> MAKKTSSKGKLPPRVPNLIPYVGSFVSFAKNPVQFIIDNSKKYGDVFTATILGKEMTFLNHPKILDTFFKATDNELSLRDVYRFMRPVFGTGVVYDADSTERMMEQVKFVSSGLTTARFRVFVDIFEDEIAHKVKELGPEGTVDVAELMADLIIFTASRCLLGDEVRQYLSEKNLGKLYHDIDDGISPLSFFYPSLPAPKRDKARKAVGEIFQELLDKRREEHKKHPERLLDESKMDVVDHLLTQKYKDGQELTDVHRIGILIAGLFAGQHTSSITSSWTLMNVISNKKVLEKVRKEQEEIMGSDKVLDYDKVMKMDYLEACMKEALRMYPPLIMIMRMARKPRECEQYIIPKGNILVVSPSVAGRCTDTYTNPDVFDPERLTERKEHEKFKYGAVPFGAGRHKCIGENFALLQVKSIISILLRYFDMEYIGKIPDPSYTSLVVGPSPPTRMR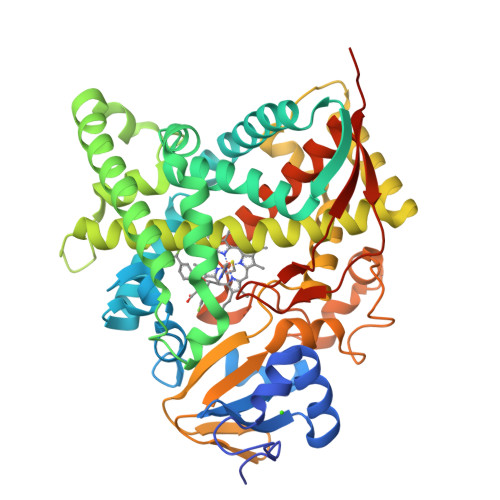YKLRKQQHHHHHH> PLLQAAKGLA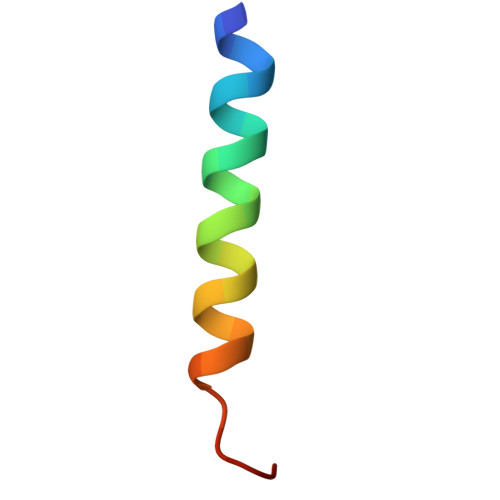GAVSELLRSAQPASA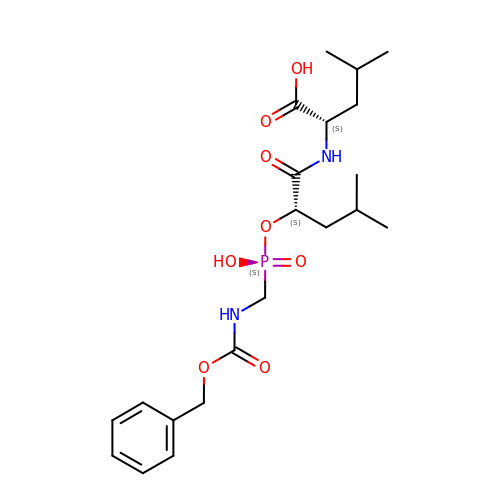N-[(2R,4S)-4-hydroxy-2-(2-methylpropyl)-4-oxido-7-oxo-9-phenyl-3,8-dioxa-6-aza-4-phosphanonan-1-oyl]-L-leucine | C21 H33 N2 O8 P | WPUXZWKBJRFUJC-ROUUACIJSA-N> AMGSSVKPIPVDLSERSTRLATVDSPGVFRVAVSSMISPLETMKGYGPVLSYIEQQTGRKVELVQRRTYREVNELIRENKIDLAFICTYSFVEAELFGARPVAVPQVEGNPYAQAVVITRRDSGINSLEELRNKRFAFTDPMSFSGHIALRGELVKVDRTPETFFASTFYTYSHDNSLRAV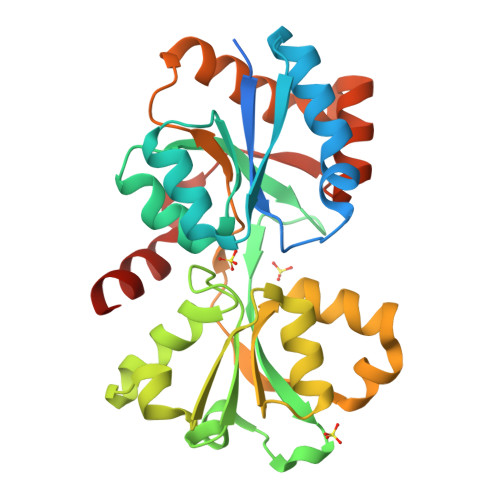YDGIVDGATIDSLVFRSSNILYPEIGAALQVVHVSPLVGAPPVVVSPGLSEEDYQLIRRAFLNMHNEPLGKQALDTLFIDRFVMVNSGHYDYIREIAGKIEVVE> ICLQKTTSTILKPRLISYTLPINTREGVCITDPLLAVDNGFFAYSHLEKIGSCTRGIAKQRIIGVGEVLDRGDKVPSMFMTNVWTPPNPSTIHHCSSTYHEDFYYTLCAVSHVGDPILNSTSWTESLSLIRLAVRPKSDSGDYNQKYIAITKVERGKYDKVMPYGPSGIKQGDTLYFPAVGFLPRTEFQYNDSNCPIIHCKYSKAENCRLSMGVNSKSHYILRSGLLKYNLSLGGDIILQFIEIADNRLTIGSPSKIYNSLGQPVFYQASYSWDTMIKLGDVDTVDPLRVQWRNNSVISRPGQSQCPRFNVCPEVCWEGTYNDAFLIDRLNWVSAGVYLNSNQTAENPVFAVFKDNEILYQVPLAEDDTNAQ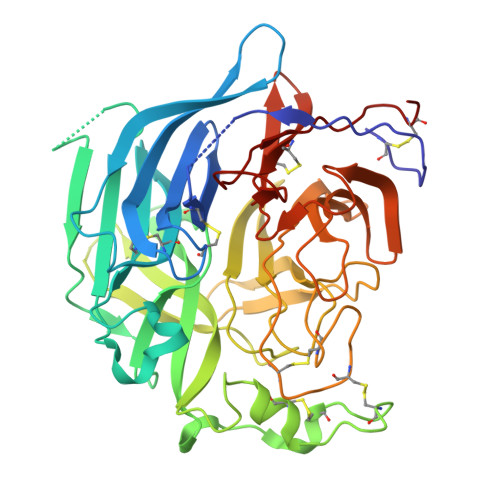KTITDCFLLENVIWCISLVEIYDTGDSVIRPKLFAVKIPAQCSE> GEFAQECQNLEVERQRRLERIKQKQSQLQELILQQIAFK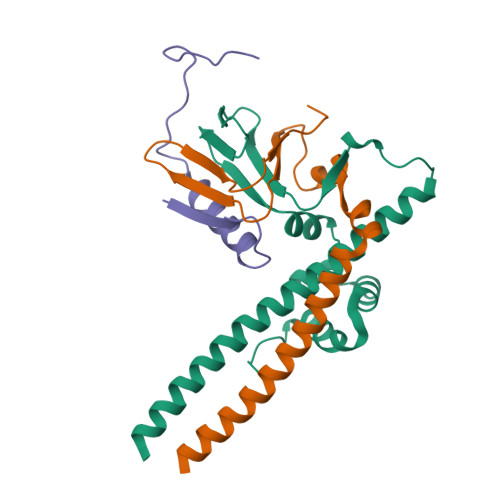NLVQRNRHAEQQASRPPPPNSVIHLPFIIVNTSKKTVIDCSISNDKFEYLFNFDNTFEIHDDIEVLKRMGMACGLESGSCSAEDLKMARSLVPKALEPYVTEMAQGTVGGVFITTA;> GSHMGGRLEGLTQDLRQLQESEQQLDHLMNICTTQLRLLSEDTDSQRLAYVTCQDLRSIADPAEQMVMVIKAPPETQLQAVDSSENFQISLKSKQGPIDVFLCPEE;> SRILVSIGESFGTSEKFQKINQMVCNSDRVLKRSAEGSNPPKPLKK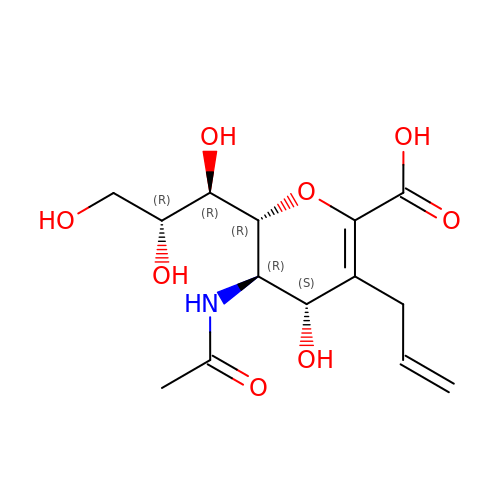5-acetamido-2,6-anhydro-3,5-dideoxy-3-prop-2-en-1-yl-D-glycero-D-galacto-non-2-enonic acid | C14 H21 N O8 | OXBQHTTZDDRTNB-BZNQNGANSA-N VACV protein A49 prevents translocation of NF-κB to the nucleus by sequestering cellular β-TrCP, a protein required for the degradation of the inhibitor of κB. Unexpectedly, the structure showed that A49 possesses a Bcl-2-like fold despite not sharing sequence identity with known cellular or poxvirus Bcl-2 family proteins. Strikingly, despite a lack of sequence conservation with known family members, A49 adopts the Bcl-2 family protein fold comprising five α-helices wrapped around a central helix, α5 (45). The A49 structure shows that A49 lacks a surface groove compatible with binding BH3 peptides and is unable to bind the proapoptotic proteins Bax or Bak.

A truncated form of A49 lacking the N-terminal 12 amino acids (A49 Δ12) was thus expressed and purified. It crystallized readily in two distinct conditions, and diffraction data were recorded to 1.8–1.9 Å resolution (A49 Δ12 ammonium sulfate and A49 Δ12 sodium malonate). Residues 13–17 adopt three distinct conformations in the 10 A49 Δ12 molecules observed in the two crystal forms (inset) and are disordered in one of the two molecules of A49 Δ12 per asymmetric unit in crystals grown in the sodium malonate condition. In four of the eight molecules of A49 Δ12 grown in the ammonium sulfate condition and both molecules of A49 Δ12 grown in the sodium malonate condition, a single residue (Gly) of the C-terminal purification tag is observed; in the structure of full-length A49, the final two residues (161 and 162) and the purification tag were not ordered and could not be modeled. Visual inspection of the structures of A49 Δ12 and full-length A49 showed that, in all cases, two molecules of A49 self-associate via an interaction of helices α4 and α6 (the “4-6 face”). In the structure of full-length A49 this interaction is formed by crystallographic 2-fold symmetry, whereas in the structures of A49 Δ12 the interaction is formed by pseudo-2-fold non-crystallographic symmetry. In the structures of A49 Δ12 salt bridges Arg136–Asp92 and Lys103–Asp139 are formed, although these bonds are not symmetric and thus formed only once per pair of A49 molecules. In A49 Δ12 hydrogen bonds are formed between the side chains of Asn88 and Tyr102 and the carbonyl oxygens of Thr128 and Val95, respectively, and between the side chains of Arg136 and Asn96, although again these interactions often occur only once per pair of A49 molecules. Additionally, we observed that A49 crystallized much more readily upon removal of residues 1–12.

>MVLGYVSDMHTELASISQLVIAKIETIDNDILNKDIVNFIMCRSNLDNPFISFLDTVYTIIDQENYQTELINSLDDNEIIDCIVNKFMSFYKDNLENIVDAIITLKYIMNNPDFKTTYAEVLGSRIADIDIKQVIRENILQLSNDIRERYLGSKHHHHHH[2x]> MLEARLEQASLLKRVVDAIKDLVQDCNFDCNDSGIALQAMDNSHVALVSMLLKAEGFSPYRCDRNIALGINLVSLTKVLRAAQNEDILTLKADDSPDAVNLMFESAETDRISEYDIKLMDIDQEHLAIPETEYAATVEMPSAEFQRICRDLNALSESVVIEATK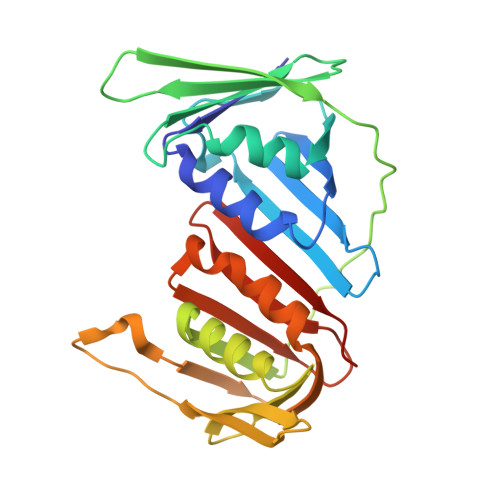EGVKFSCQGDIGSGSVTIRQHTSVDKPEQNVSIALSEPVALTFSLKYLVNFCKATSLSSKVTLCLSQEVPLLVEYGLGSGHLRFYLAPKIGDE>[2x]MKKIQTPNAKGEVRIIAGLWRGRKLPVLNSEGLRPTGDRVKETLFNWLMPYIHQSECLDGFAGSGSLGFEALSRQAKKVTFLELDKTVANQLKKNLQTLKCSSEQAEVINQSSLDF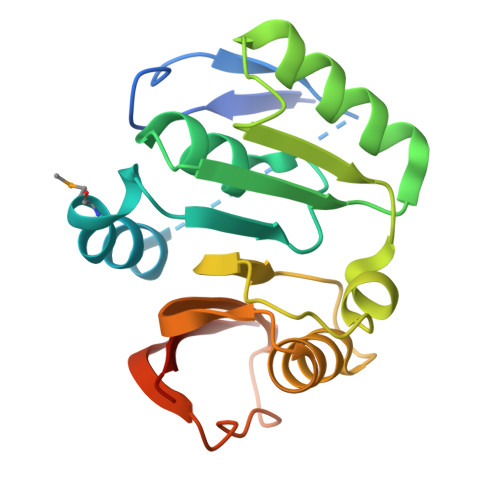LKQPQNQPHFDVVFLDPPFHFNLAEQAISLLCENNWLKPNALIYVETEKDKPLITPENWTLLKEKTTGIVSYRLYQNLEHHHHHH>[2x]MNITGKGAYDTGTYANLFQRSGYREDEIKARLEQTWNDLFYGDEHTRIYYPVGDDKGYMLDTGNDDVRSEGMSYGM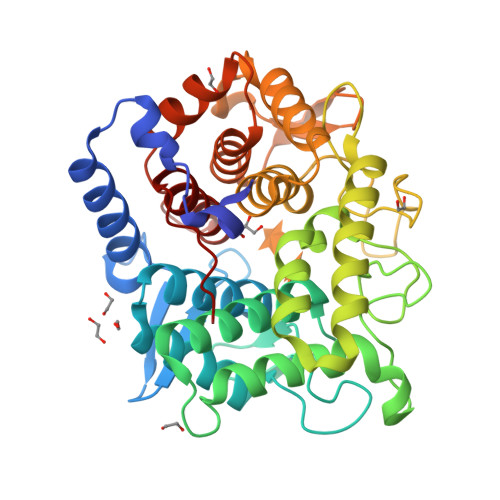MMAVQMDKKHEFDRLWNYAYTYMQHTEGRYKDYFAWHCKPDGTRLSPGPAPDGEEFFAMALFFASNRWGDGPAPYDYQAQARKILHACLHQGEQGEGDPMWEPSNRLIKFIPELPFSDPSYHLPHFYELFAQYANEQDRTFWKEAAEASRAYLRTACHPVTGLSPEYANYDGTPAPVQLHGDFRHFYSDAYRVAANVALDWEWFRKDPWQVQQSNRIQAFFSDIDVSDYRRYTIEGEPFNEPAAHPVGLLATNAMASLAADGPDADSFVKRFWNTPLRQGKRRYYDNCLYFFTMLALSGNYRVYQQ> SENSLEIEELARFAV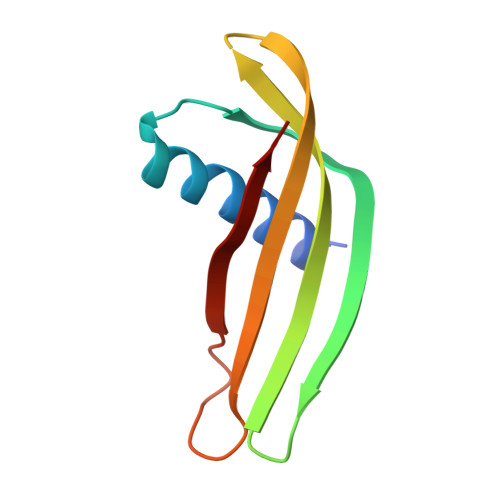DEHNKKENALLEFVRVVKAKEQERNSIFEEFTMYYLTLEAKDGGKKKLYEAKVWVKRDLVFGGPENFKELQEFKPV>NLVFSDGYVVKETIGVGSYSECKRCVHKATNMEYAVKVIDKSKRDPSEEIEILLRYGQHPNIITLKDVYDDGKHVYLVTELMRGGELLDKILRQKFFSEREASFVLHTIGKTVEYLHSQGVVHRDLKPSNILYVDESGNPECLRICDFGFAKQLRAENGLLMTPCYTANFVAPEVLKRQGYDEGCDIWSLGILLYTMLAGYTPFANGPSDTPEEILTRIGSGKFTLSGGNWNTVSETAKDLVSKMLHVDPHQRLTAKQVLQHPWVTQKDKLPQSQLSHQDLQLVKGAMA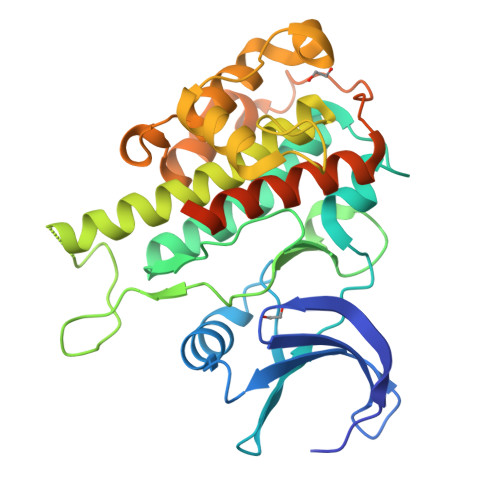ATYSALNSSKPTPQLKPIESSILAQRRVRKLPSTTL[2x]> DPLAWDNHYGTQIPKEEWKSQEKSPEKTAFKKKDTILSLNACESNHAIAAINEGQNKPEIEVTWAKQGRTERLCSQNPPVLKRHQREITRTTLQSDQEEIDYDDTISVEMKKEDFDIYDEDENQSPRSFQKKTRHYFIAAVERLWDYGMSSSPHVLRNRAQSGSVPQFKKVVFQEFTDGSFTQPLYRGELNEHLGLLGPYIRAEVEDNIMVTFRNQASRPYSFYSSLISYEEDQRQGAEPRKNFVKPNETKTYFWKVQHHMAPTKDEFDCKAWAYSSDVDLEKDVHSGLIGPLLVCHTNTLNPAHGRQVTVQEFALFFTIFDETKSWYFTENMERNCRAPCNIQMEDPTFKENYRFHAINGYIMDTLPGLVMAQDQRIRWYLLSMGSNENIHSIHFSGHVFTVRKKEEYKMALYNLYPGVFETVEMLPSKAGIWRVECLIGEHLHAGMSTLFLVYSNKCQTPLGMASGHIRDFQITASGQYGQWAPKLARLHYSGSINAWSTKEPFSWIKVDLLAPMIIHGIKTQGARQKFSSLYISQFIIMYSLDGKKWQTYRGNSTGTLMVFFGNVDSSGIKHNIFNPPIIARYIRLHPTHYSIRSTLRMELMGCDLNSCSMPLGMESKAISDAQITASSYFTNMFATWSPSKARL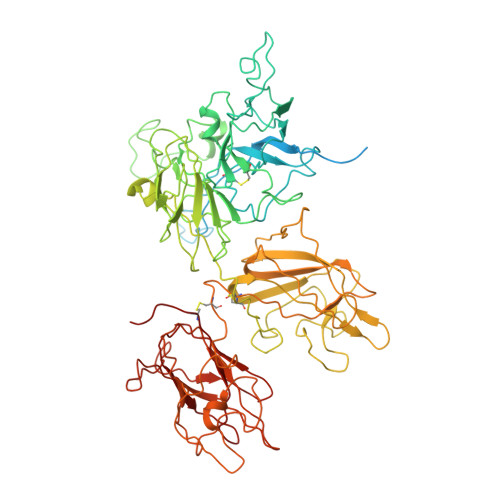HLQGRSNAWRPQVNNPKEWLQVDFQKTMKVTGVTTQGVKSLLTSMYVKEFLISSSQDGHQWTLFFQNGKVKVFQGNQDSFTPVVNSLDPPLLTRYLRIHPQSWVHQIALRMEVLGCEAQDLY> GSHHHHHHSQDPMQAAQETKQKLTSCLARRYNAEQKLLDLSALGTDETLSSLGSFNNQSLAEKSFKALMHLVSNEYKDPEQKNEAIQAVSLARNDILDVGQVYSLAVTLPRLRRLDLSGNNLENLSKISKWQQEFRFLEELHLTGNPVTTLPNYATEIKKWFPSLQILDGQQIRTPQEAA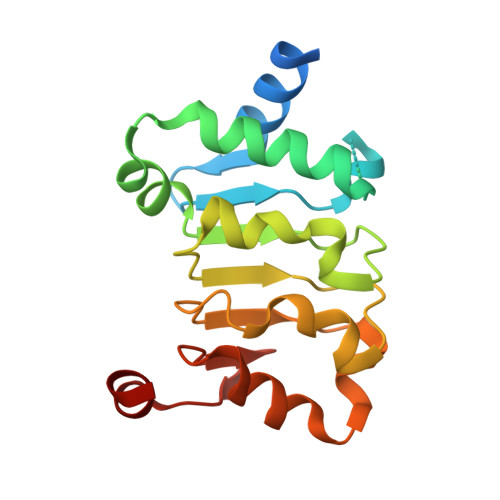ESL>[4x]LAAVSVDCSEYPKPACPKDYRP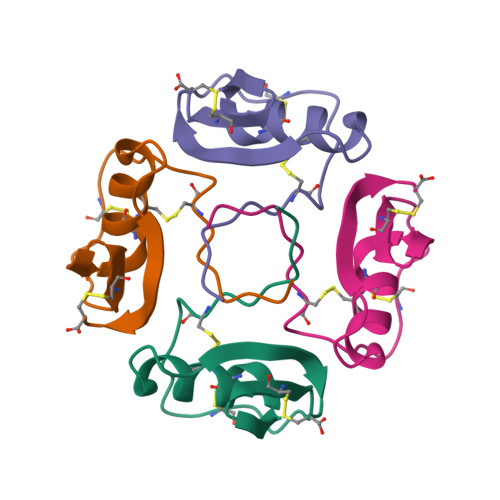VCGSDNKTYSNKCNFCNAVVESNGTLTLNHFGKC>MAVNFYDVAYDLENALRGSEEFTRLKNLYDEVNADESAKRMFENFRDVQLRLQQKQMAGEEITQEEVTQAQKTVALVQQHEKISQLMEAEQRMSMLIGEL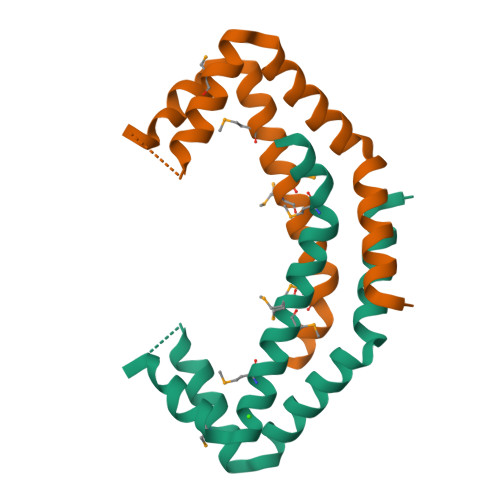NKIIMKPLEELYGSVEG[2x]> AATTGYDAVDDLLHYHERGNGIQINGKDSFSNEQAGLFITRENQT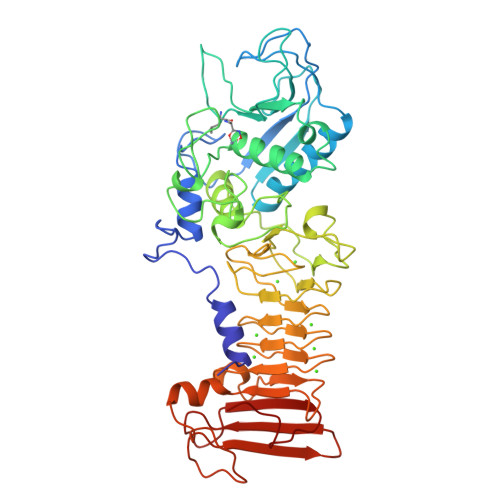WNGYKVFGQPVKLTFSFPDYKFSSTNVAGDTGLSKFSAEQQQQAKLSLQSWADVANITFTEVAAGQKANITFGNYSQDRPGHYDYGTQAYAFLPNTIWQGQDLGGQTWYNVNQSNVKHPATEDYGRQTFTHEIGHALGLSHPGDYNAGEGDPTYNDVTYAEDTRQFSLMSYWSETNTGGDNGGHYAAAPLLDDIAAIQHLYGANLSTRTGDTVYGFNSNTGRDFLSTTSNSQKVIFAAWDAGGNDTFDFSGYTANQRINLNEKSFSDVGGLKGNVSIAAGVTIENAIGGSGNDVIVGNAANNVLKGGAGNDVLFGGGGADELWGGAGKDIFVFSAASDSAPGASDWIRDFQKGIDKIDLSFFDKEANSSSFIHFVDHFSGTAGEALLSYNASSNVTDLSVNIGGHQAPDFLVKIVGQVDVATDFIV>MGNKICQFKLVLLGESAVGKSSLVLRFVKGQFHEFQESTIGAAFLTQTVCLDDTTVKFEIWDTAGQERYHSLAPMYYRGAQAAIVVYDITNEESFARAKNWVKELQRQASPNIVIALSGNKADLANKRAVDFQEAQSYADDNSLLFMET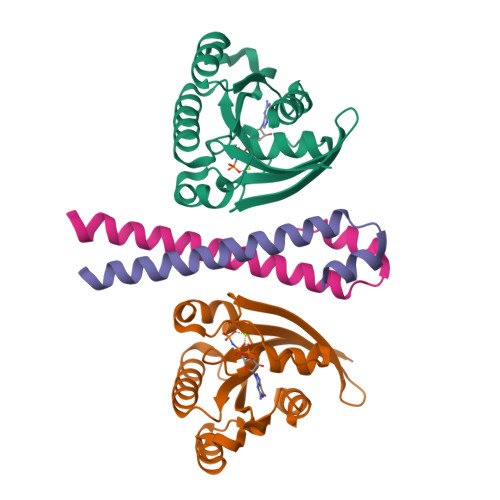SAKTSMNVNEIFMAIAKKLPKN[5x];>GPLGSAKATVEQLMFEEKNKAQRLQTELDVSEQVQRDFVKLSQTLQVQLERIRQADSLERIRAILNDTKLTDINQLPET[5x]>MKIIMFSVRDDEEAAIREWEKKTGVQVDINRLELDAETAQLTKGYDGIVIQQRSHISNPAVYETLQKNGLRQLTSRTAGYDMIDLEQASERGLVVTNVPAYSPNSVAELALTQTMRLIRNLPLFDARGAEQDFRWAGLMAREIRSLTVGIIGAGRIGGTVARLFK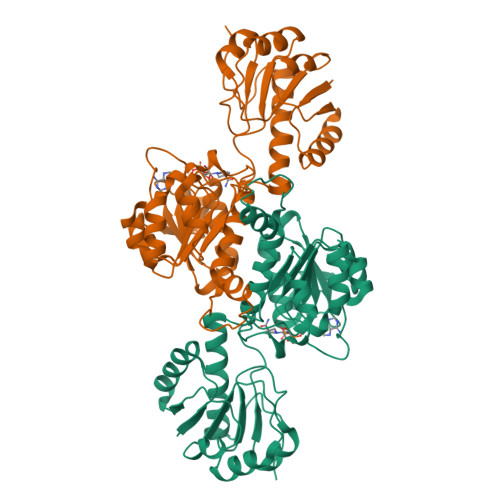ALGATVIANDIVERVELKDIVTYVSKEELLQAADVVTLHVPLMDSTTQLIDADALALMKNDAVLINASRGPVVDTDALIAALQNKQIAGAALDTLNGEEHFFNQDLCGKELPSEQLKVLRTLPNVLITPHIGFYTNKAVQNMVEISLNDVLAILKTGTSEHQLNKVAVEN[2x]> MGHHHHHHAMEGKITPVSVKKVDDKV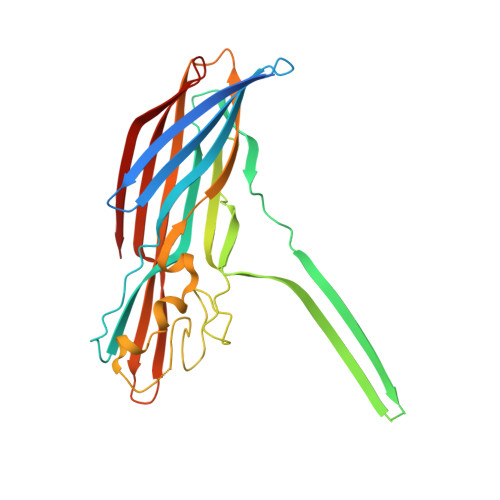TLYKTTATADSDKFKISQILTFNFIKDKSYDKDTLVLKATGNINSGFVKPNPNDYDFSKLYWGAKYNVSISSQSNDSVNVVDYAPKNQNEEFQVQNTLGYTFGGDISISNGLSGGLNGNTAFSETINYKQESYRTTLSRNTNYKNVGWGVEAHKIMNNGAGPYGRDSFHPTYGNELFLAGAQSSAYAGQNFIAQHQMPLLSRSNFNPEFLSVLSHRQDGAKKSKITVTYQREMDLYQICWNGFYWAGANYKNFKTRTFKSTYEIDWENHKVKLLDTKETENNK In Gram-positive organisms, the smaller plasmids often replicate via a rolling circle mechanism, a process mediated by a multi-functional replication initiation protein (Rep) encoded on that plasmid. The Rep proteins possess two related catalytic activities, a type-I topoisomerase-like cleavage activity in which they form a nick in the (+) strand at the origin of replication to initiate DNA synthesis, and a religation activity to join the ends of the parental strand that is displaced during replication. Despite low overall sequence identity, there is a high degree of structural conservation between the catalytic domains of the Rep proteins from these Geobacillus stearothermophilus and Staphylococcus aureus plasmids. Structure-based sequence alignment reveals the conserved residues are almost exclusively located in the β-strands containing the Rep_trans motifs, and it is likely the crescent-shaped catalytic domain represents the canonical fold for the Rep_trans protein family.

In this report we describe the structure determination of the core domain of replication initiator protein of cryptic plasmid pSTK1 (25,26) from Geobacillus stearothermophilus (RepSTK1 residues 1–269 (27), hereafter referred to as RepSTK1). This was then used to aid the structure solution of two staphylococcal Rep variants, RepDE and RepDN (containing the 21 kDa fragment of RepD fused to the 14 kDa fragment of RepE or RepN, respectively). Constructs of RepDE and RepDN spanning residues 35–314 were used for crystallisation studies, since the first 34 amino acids are predicted to be disordered and had previously been shown to be dispensable for protein function. Crystals of RepDN belong to space group I213, but the data were near perfectly twinned (refined twin fraction of 49.8%) giving an apparent space group of I4132. The twinning severely hampered experimental phasing; however, it was possible to produce some partially interpretable electron density maps using SIRAS data collected from seleno-methionine labelled crystals. Molecular replacement with the RepSTK1 coordinates was also unsuccessful, but manual docking of fragments of the RepSTK1 model into the RepDN density allowed further interpretation of the RepDN electron density maps. Crystals of both RepDE and RepDN contain two molecules per asymmetric unit as a non-crystallographic dimer and the final structural model spans residues 39–308 for all subunits. The relative orientation of the catalytic domains in RepDN is intermediate between those observed in the other two proteins. They still form a ‘horseshoe’, but are rotated 5° towards each other relative to the position in RepDE, reducing the distance between protein chains at the open end of the ‘horseshoe’ by 5 Å. The different conformations adopted by RepDE and RepDN demonstrate the catalytic domains can move relative to one another to modify the size of the cavity containing the active sites.

>MFFTTPQPELSFDAMTIVGNLNKTNAKKLSDFMSTEPQIRLWDILQTKFKAKALQEKVYIEYDKVKADSWDRRNMRVEFNPNKLTHEEMLWLKQNIIDYMEDDGFTRLDLAFDFEDDLSDYYAMTDKAVKKTIFYGRNGKPETKYFGVRDSDRFIRIYNKKQERKDNADVEVMSEHLWRVEIELKRDMVDYWNDCFNDLHILQPDWKTIERTSDRAMVFMLLNDEEEWGKLERRTKNKYKKLIKEISLIDLTDLMKSTLKANEKQLQKQIDFWQREFRFWK[2x]> VPDPRGIIINLDEGELCLNSAQCKSNCCQHDTILSLSRCALKARENSECSAFTLYGVYYKC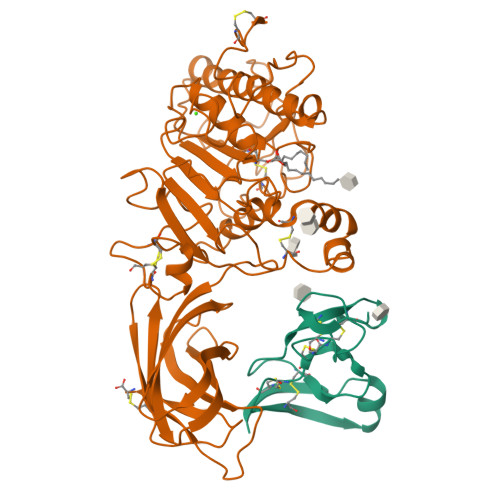PCERGLTCEGDKSLVGSITNTNFGICHNVGRSDS;> KEVCYERLGCFSDDSPWSGITERPLHILPWSPKDVNTRFLLYTNENPNNFQEVAADSSSISGSNFKTNRKTRFIIHGFIDKGEENWLANVCKNLFKVESVNCICVDWKGGSRTGYTQASQNIRIVGAEVAYFVEFLQSAFGYSPSNVHVIGHSLGAHAAGEAGRRTNGTIGRITGLDPAEPCFQGTPELVRLDPSDAKFVDVIHTDGAPIVPNLGFGMSQVVGHLDFFPNGGVEMPGCKKNILSQIVDIDGIWEGTRDFAACNHLRSYKYYTDSIVNPDGFAGFPCASYNVFTANKCFPCPSGGCPQMGHYADRYPGKTNDVGQKFYLDTGDASNFARWRYKVSVTLSGKKVTGHILVSLFGNKGNSKQYEIFKGTLKPDSTHSNEFDSDVDVGDLQMVKFIWYNNVINPTLPRVGASKIIVETNVGKQFNFCSPETVREEVLLTLTPC> QEKLGDICFSLRYVPTAGKLTVVILEAKNLK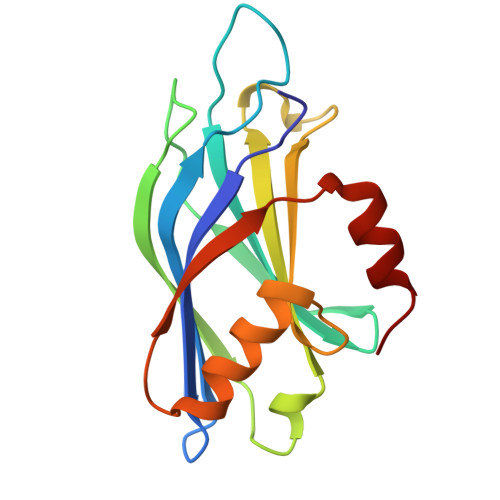KMDVGGLSDPYVKIHLMQNGKRLKKKKTTIKKNTLNPYYNESFSFEVPFEQIQKVQVVVTVLDYDKIGKNDAIGKVFVGYNSTGAELRHWSDMLANPRRPIAQWHTLQVEEEVDAMLAVKK> MSTVKAPTLPASIFRAYDIRGVVGDTLTAETAYWIGRAIGSESLARGEPCVAVGRDGRLSGPELVKQLIQGLVDCGCQVSDVGMVPTPVLYYAANVLEGKSGVMLTGSHNPPDYNGFKIVVAGETLANEQIQALRERIEKNDLASGVGSVEQVDILPRYFKQIRDDIAMAKPMKVVVDCGNGVAGVIAPQLIEALGC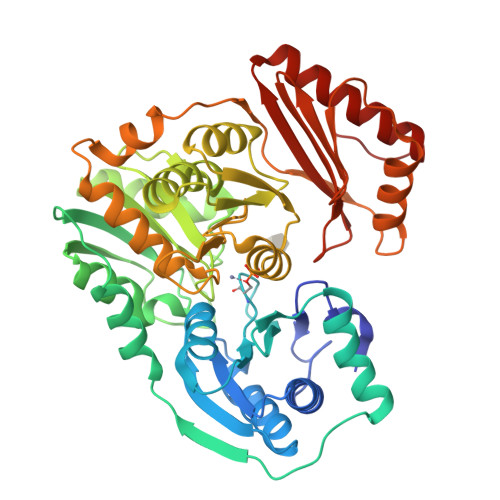SVIPLYCEVDGNFPNHHPDPGKPENLKDLIAKVKAENADLGLAFDGDGDRVGVVTNTGTIIYPDRLLMLFAKDVVSRNPGADIIFDVKCTRRLIALISGYGGRPVMWKTGHSLIKKKMKETGALLAGEMSGHVFFKERWFGFDDGIYSAARLLEILSQDQRDSEHVFSAFPSDISTPEINITVTEDSKFAIIEALQRDAQWGEGNITTLDGVRVDYPKGWGLVRASNTTPVLVLRFEADTEEELERIKTVFRNQLKAVDSSLPVPF>[2x]HHHHGSRFLIRLVPEDKDRAFKVPYNHQYYLQGLIYNAIKSSNPKLATYLHEVKGPKLFTYSLFMAEKREHPKGLPYFLGYKKGFFYFSTCVPEIAEALVNGLLMNPEVRLWDERFYLHEIKVL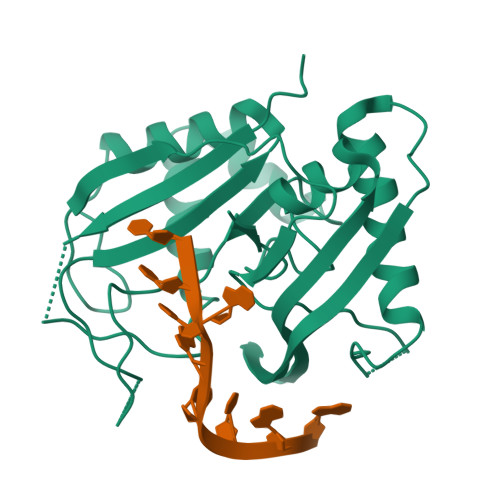REPKKFNGSTFVTLSPIAVTVVRKGKSYDVPPMEKEFYSIIKDDLQDKYVMAYGDKPPSEFEMEVLIAKPKRFRIKPGIYQTAWHLVFRAYGNDDLLKVGYEVGFGEKNSLGFGMVKVEGNKTTKEAEEQEKITFNSREELKTGV> MNDIIINKIATIKRCIKRIQQVYGDGSQFKQDFTLQDSVILNLQRCCEACIDI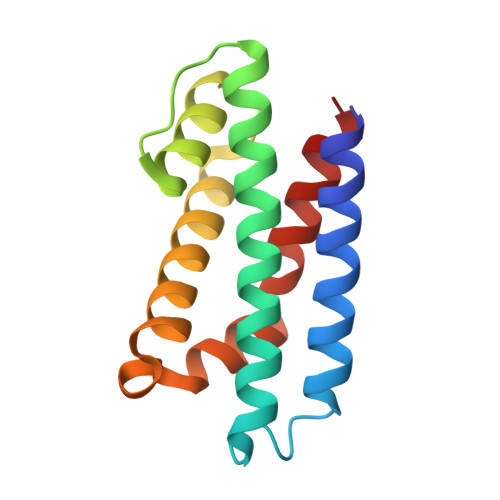ANHINRQQQLGIPQSSRDSFTLLAQNNLITQPLSDNLKKMVGLRNIAVHDAQELNLDIVVHVVQHHLEDFEQFIDVIKAE2-amino-7-fluoro-5-oxo-5H-chromeno[2,3-b]pyridine-3-carboxamide | C13 H8 F N3 O3 | 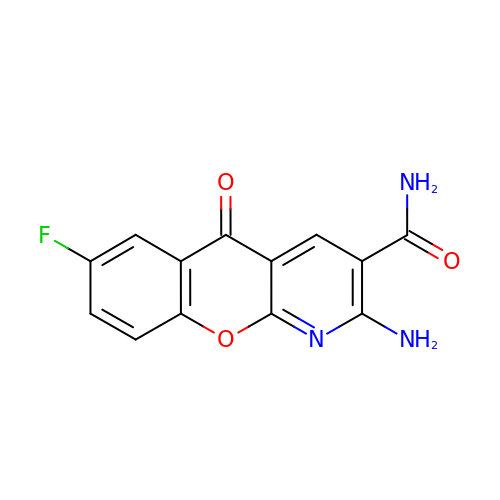GCHMLYYPYFXLQB-UHFFFAOYSA-N> MVHESNPNDYAAGDAGNASGRYTTGSNGIPPMLPSVRSVWLDAFNDPVAGISAYTPCVHTCNLFGDGENRLVIADEDRKLKIWKGTQKASEHPLLDTPVAICSYISENTAPRLPALAVAAGSHIYIYRNLRPYYKFVLPPENVNTEEQDIWQKVMEGEIVIGEAVAQLTRLQVRAGDAGVVLQTRSLQLMNIGDPDAKMAFVEHWQGQPLVATTVITCMDVVKQAIDEPDAVSCLVVGTESGR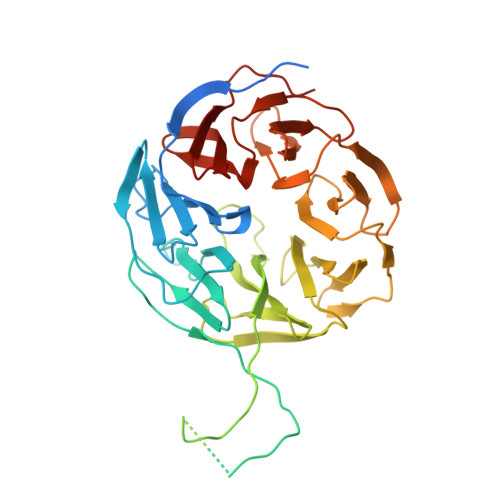ILILNPAGTAIVKNIWVGITPAMIAVQGELDVGYRITVAGRDGKLYHIRNGELSQTIIQLEAQPVGLVRLAKHVAVGCMNDVVHAYTPTGHKSWSLYLPCHILAMQRMEVTGQRNTKALIVALSNGEVRVYNEKLLVSVHVSPNPVTALWFGRYGREDNTLLAITKSGALDIKMLPRTANLE>ESQLDLRVQELLKLICNVQTMEEMMIEMKYDTKRAPLGKLTVAQIKAGYQSLKKIEDCIRAGQHGRALVEACNEFYTRIPHDFGLSIPPVIRTEKELSDKVKLLEALGDIEIALKLVKSERQGLEHPLDQHYRNLHCALRPLDHESNEFKVISQYLQSTHAPTHKDYTMTLLDVFEVEKEGEKEAFREDLPNRMLLWHGSRLSNWVGILSHGLRVAPPEAPITGYMFGKGIYFADMSSKSANYCFASRLKNTGLLLLSEVALGQCNELLEANPKAQGLLRGKHSTKGMGKMAPSPAHFIT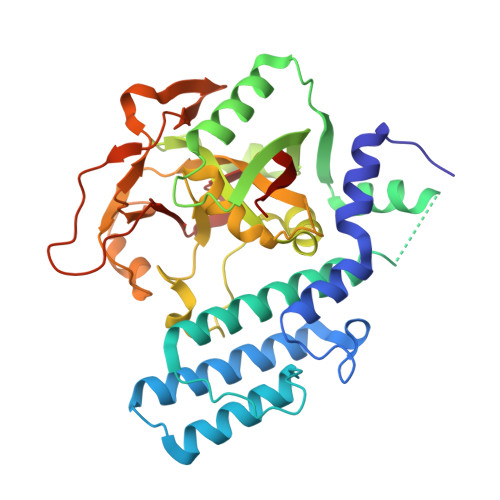LNGSTVPLGPASDTGILNPEGYTLNYNEFIVYSPNQVRMRYLLKIQFNFLQ[2x]> YVDYKDDDDKEFEVCSEQAETGPCRAGFSRWYFDVTEGKC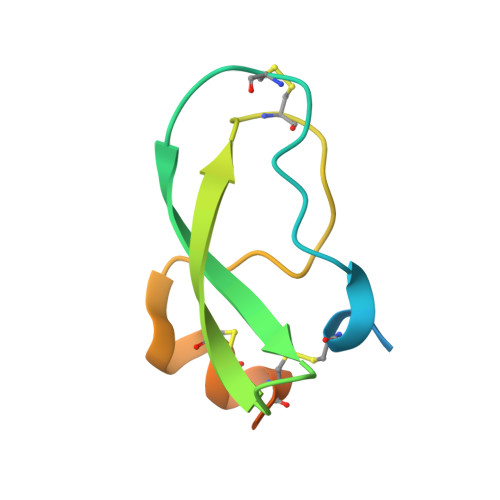APFVYGGCGGNRNNFDTEEYCMAVCGSAIPRHHHHHHAAAN> MASQGPGEVVLLDFAAAGGE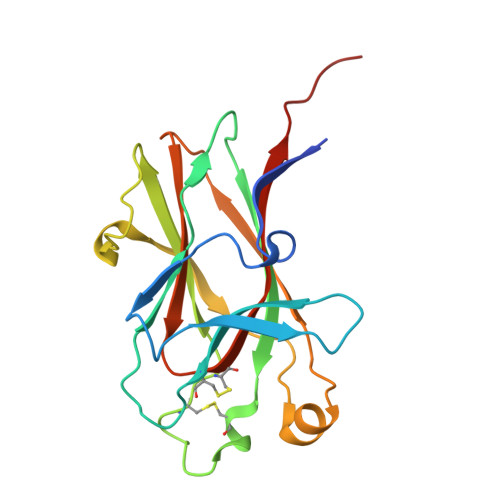LGWLTHPYGKGWDLMQNIMNDMPIYMYSVCNVMSGDQDNWLRTNWVYRGEAERIFIELKFTVRDCNSFPGGASSCKETFNLYYAESDLDYGTNFQKRLFTKIDTIAPDEITVSSDFEARHVKLNVEERSVGPLTRKGFYLAFQDIGACVALLSVRVYYKKAHHHHHH> KNTASRSAASVPANEQISQLASLVAA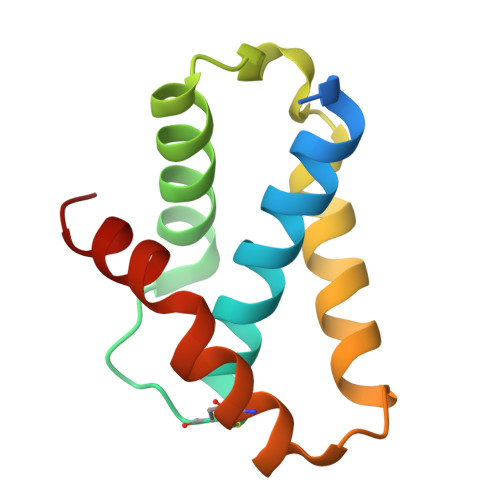SKYLRVQCERSDLPDDGTILKTAVNVAVQKGWDTGRYQSLPQLSENLYQGLLKDGTPKATQCSSFNRTMTPFLDAMRTVR>[2x]MTSRIRFLMCPPDHYDVDYVINPWMEGNIHKSSRDRAVEQWQGLYQILKEHAIVDLVTPQKGWPDLVFTANAGLVLGDNVVLSRFLHKERQGEEPYFKEWFEGNGYTVYELPKDLPFEGAGDALLDREGRWLWAGYGFRSELDSHPYLAKWLDIEVLSLRLIDERFYHLDTCFCPLANGYLLYYPGAFDSYSNRLIEMRVAPEKRIAIAEADAVNFACNTVNVESIVIMNKASDALKQSLTGVGFQVLETPLTEFLKAGGAAKCLTLRVTEPVRDEVHANVYVESRIIRIEGHLLDSGLINRALDMIVDTGGSFQVLNFNLGEQRQSTSAAEVKVSAPSHEVMEEIISLLIDLGAVDLPQDERDAKLEPVIQDGVAPDDFYVSTIYPTEVRINGQWIKVENQRMDGAIAITQTPNGLLAQCKILRDLKAGEQVIVDVLGIRTIRKTESREQRNTQEFSFMSGGVSSERRVELVVEQVAWELRKIRDAGGKVVVTAGPVVI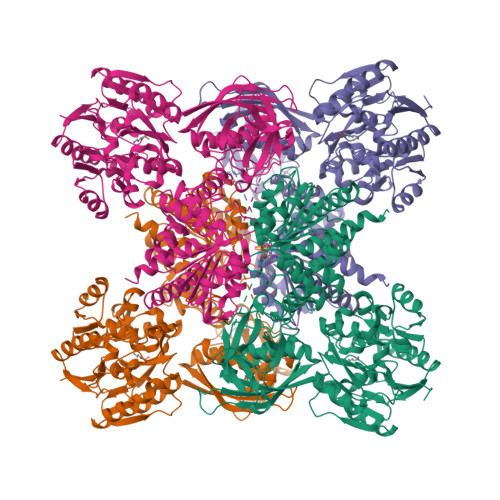HTGGGEHLSRLIREGYVQALLGGNAIAVHDIEQNMMGTSLGVDMKRGVAVRGGHRHHLKVINTIRRHGSIAKGVESGIIRSGVMYECVRNQIPFVLAGSIRDDGPLPDTQMDLIKAQEEYAKHLEGAEMILMLSSMLHSIGVGNMTPAGVKMVCVDINPAVVTKLSDRGSIESVGVVTDVGLFLSLLTQQLDKLTSPYVSKVG>[4x]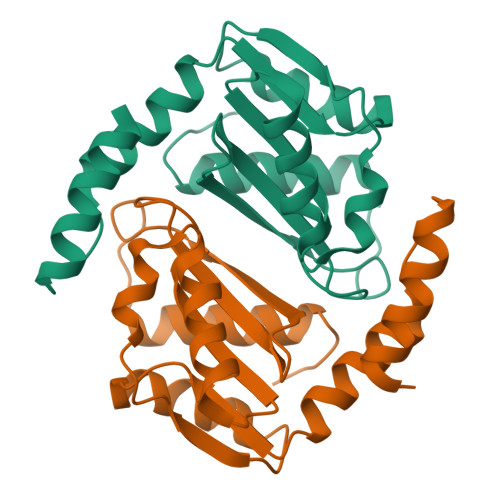MNIENTIKSAYEESLNNARFGDKIEEIDAIQSTIKSAKNVTVATSNEKKFKVVSDIISRITDANISMLEIPTNSADLTRMPALNKGLIAVDSSDADLIITRGRLGIPGSGSLLLIMDKKGRILTGSVSPSSIIHKNPIDKTVELELITALERIGIVVKKLEHHHHHH> SYYSTLQCRNNHGHCRRLCFHGEQWIGNCNGRHQHCCK

Defensins, a family of cysteine-rich cationic host defence peptides, are a major component of the innate immune systems of all plant and animal species, however crocodilian defensins are poorly characterised. We now report the functional and structural characterisation of Crocodylus porosus β-defensin 13 (CpoBD13). We now show that the saltwater crocodile defensin CpoBD13 harbors potent antifungal activity that is mediated by a pH-dependent membrane-targeting action. CpoBD13 binds the phospholipid phosphatidic acid (PA) to form a large helical oligomeric complex, with specific histidine residues mediating PA binding.

To understand the structural basis of CpoBD13 activity, we determined its atomic structure using X-ray crystallography. A single copy of CpoBD13 was found in the asymmetric unit, with clear and continuous density observed for the entire protein chain. CpoBD13 adopts a fold comprising the family-defining structural elements observed in mammalian β-defensins comprising a single α-helix and a three-stranded β-sheet, which are connected via three disulphide bonds. A Dali analysis of CpoBD13 revealed that human β-defensin-2 (HBD-2) is the closest structural homologue in the Protein Data Bank (PDB), with a rmsd of 0.8 Å (Z-score 6.2) over 40 Cα atoms, and a peptide sequence identity of 26% (only I26 and K38 are conserved in addition to the cysteine residues that form the structurally critical disulphide bonds). An overlay of the two defensin structures revealed that residue H35 of CpoBD13 was located in the same position as the key lipid binding residue K36 in HBD-2. We surmised that if the activity of CpoBD13 is as conserved with HBD-2 as its tertiary structure, the co-localisation of these amino acids could indicate that histidine may play a role in CpoBD13–lipid interactions. Our findings reveal that despite limited primary sequence identity, the three-dimensional structure of CpoBD13 bears a striking resemblance to HBD-2, suggesting strong evolutionary conservation of the β-defensin structure between humans and reptiles.>[6x]GSHMENREPPLLPARWSSAYVSYWSPMLPDDQLTSGYCWFDYERDICRIDGLFNPWSERDTGYRLWMSEVGNAASGRTWKQKVAYGRERTALGEQLCERPLDDETGPFAELFLPRDVLRRLG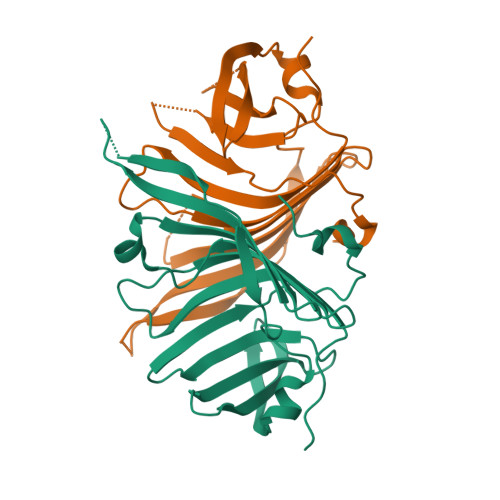ARHIGRRVVLGREADGWRYQRPGKGPSTLYLDAASGTPLRMVTGDEASRASLRDFPNVSEAEIPDAVFAAKR>[2x]MPKEKPHVNIVFIGHVDHGKSTTIGRLLYDTGNIPETIIKKFEEMGEKGKSFKFAWVMDRLKEERERGITIDVAHTKFETPHRYITIIDAPGHRDFVKNMITGASQADAAVLVVAATDGVMPQTKEHAFLARTLGIKHIIVTI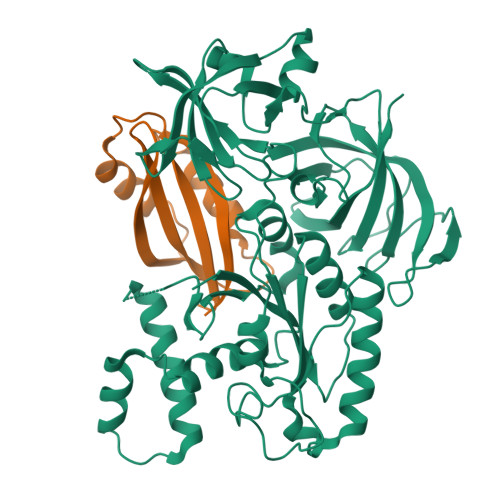NKMDMVNYDQKVFEKVKAQVEKLLKTLGYKDFPVIPTSAWNGDNVVKKSDKMPWYNGPTLIEALDQIPEPEKPIDKPLRIPIQDVYSIKGVGTVPVGRVETGKLKVGDVVIFEPASTIFHKPIQGEVKSIEMHHEPLQEALPGDNIGFNVRGVSKNDIKRGDVAGHTDKPPTVVRTKDTFKAQIIVLNHPTAITVGYSPVLHAHTAQIPVRFEQILAKVDPRTGNIVEENPQFIKTGDSAIVVLRPMKPVVLEPVKEIPQLGRFAIRDMGMTIAAGMVISIQKGEHHHHHH;>MSDFNLVGVIRVMPTDPDVNLDELEEKLKKVIPEKYGLAKVEREPIAFGLVALKFYVLGRDEEGYSFDEVAEKFEEVENVESAEVETVSRI[2x]> RTFRQ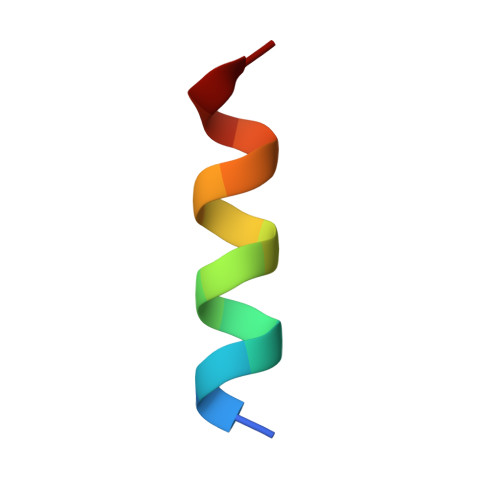VQSSISDFYD>[2x]TQFDKQYNSIIKDIINNGISDEEFDVRTKWDSDGTPAHTLSVISKQMRFDNSEVPILTTKKVAWKTAIKELLWIWQLKSNDVNDLNMMGVHIWDQWKQEDGTIGHAYGFQLGKKNRSLNGEKVDQVDYLLHQLKNNPSSRRHIT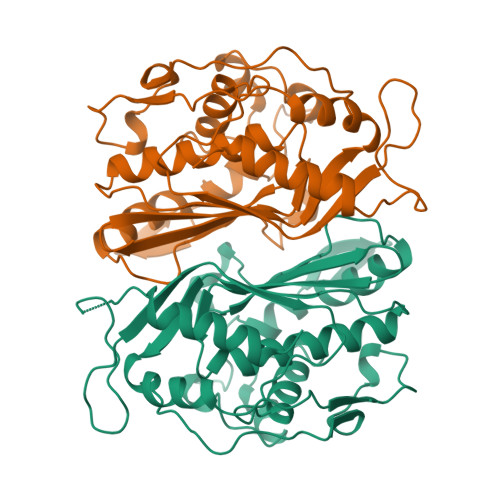MLWNPDELDAMALTPCVYETQWYVKHGKLHLEVRARSNDMALGNPFNVFQYNVLQRMIAQVTGYELGEYIFNIGDCHVYTRHIDNLKIQMEREQFEAPELWINPEVKDFYDFTIDDFKLINYKHGDKLLFEVAV>[6x]GGGGGGMKRFYIANEDE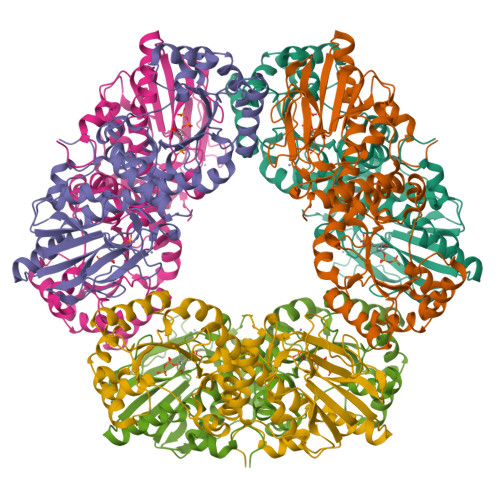IKAGKTTDVYFLRTKKILEVKNIRKKVLADVTTTSLPNNWRWGVLVGVEEVAKLLEGIPVNVYAMPEGTIFHPYEPVLQIEGDYADFGIYETALLGMLSQASGIATAALRIKIAAKFKPVYSFGIRHMHPAIAPMIDRAAFIGGCDGVSGVLGAEMMGEKAVGTMPHALIITVGDQVKAWKYFDEVIEEEVPRIALVDTFYDEKVEAVMAAEALGKKLFAVRLDTPSSRRGNFRKIIEEVRWELKVRGYDWVKIFVSGGLDEEKIKEIVDVVDAFGVGGAIASAKPVDFALDIVEVEGKPIAKRGKLSGRKQVYRCENGHYHVVPANKKLERCPVCNAKVEPLLKPIIENGEIVVEFPKAREIREYVLEQAKKFNLEI>[2x]GHMAPIKVI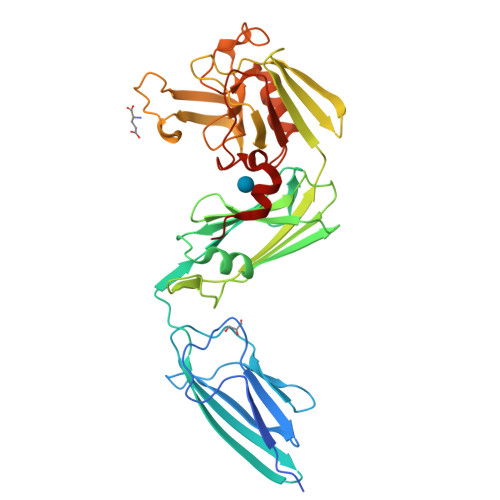ADKGTPFADLLVPKLTASVTDGAVGVTVDAPVSVTAADGVLAAVTMVNDNGRPVAGRLSPDGLRWSTTEQLGYNRRYTLNATALGLGGAATRQLTFQTSSPAHLTMPYVMPGDGEVVGVGEPVAIRFDENIADRGAAEKAIKITTNPPVEGAFYWLNNREVRWRPEHFWKPGTAVDVAVNTYGVDLGEGMFGEDNVQTHFTIGDEVIATADDNTKILTVRVNGEVVKSMPTSMGKDSTPTANGIYIVGSRYKHIIMDSSTYGVPVNSPNGYRTDVDWATQISYSGVFVHSAPWSVGAQGHTNTSHGCLNVSPSNAQWFYDHVKRGDIVEVVNTVGGTLPGIDGLGDWNIPWDQWRAGNAKA>MFHTVDVKGVQTRYFDDGQDKDPILLIHGGHFGFFIPVGIESWGNVLEDFGEYGRVLAVDKLGQGETGLPLNDEDWTVDAVAEHVANFATQLGLKNLTLVGHSRGGMTAVL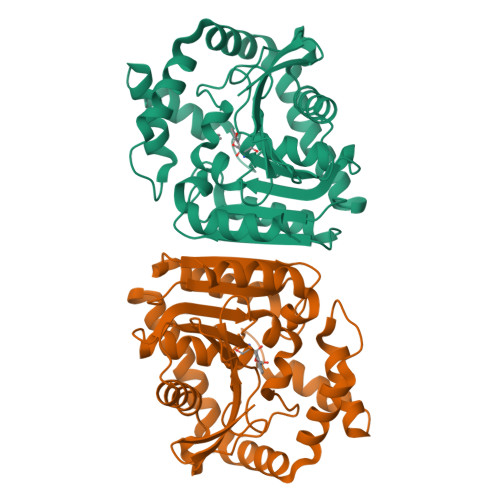LALKYPEMVKKLVIISSATAAPAPPVGTDMDFYERVERTAPGGSAELIRHYHAAQAVNEGDLPEDYIGIATKWLESEKQLDAVAGYARNAEEHWLPSLSEGRRWVQERLADAGIPVPTLVVWGVNNRSAPVSMGKGLFDLIAANTLDSSLYLINNAGHHVFSDQREKFNAAVGAFISL[4x]> GSHM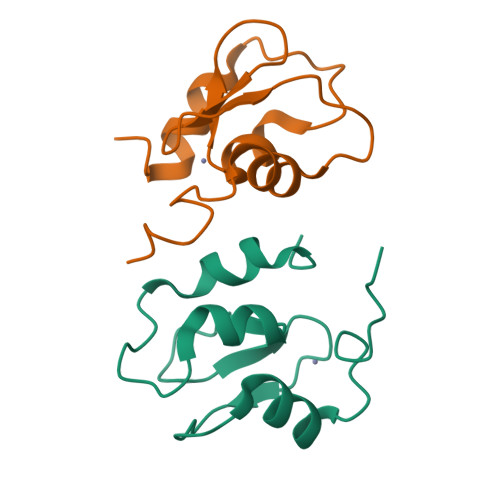KTCVPADINKEEEFVEEFNRLKTFANFPSGSPVSASTLARAGFLYTGEGDTVRCFSCHAAVDRWQYGDSAVGRHRKVSPNCRFINGFYLE>MNHLISGFENFEKKINYRFKNKAYLLQAFTHASYHYNTITDCYQRLEFLGDAILDYLITKHLYEDPRQHSPGVLTDLRSALVNNTIFASLAVKYDYHKYFKAVSPELFHVIDDFVQFQLEKNEMQGMDSELRRSEEDEEKEEDIEVPKAMGDIF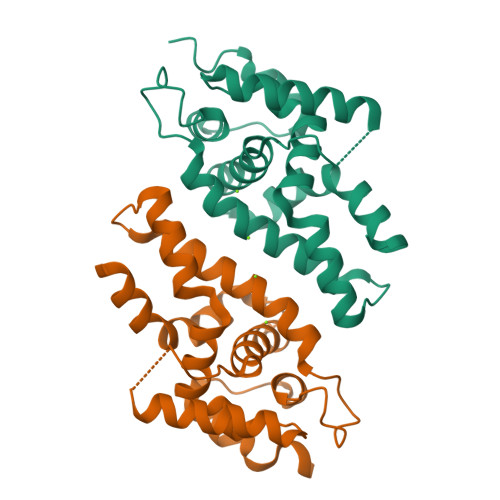ESLAGAIYMDSGMSLETVWQVYYPMMRPLIEKFSANVPRSHHHHHH[3x]>MRGSHHHHHHGSMEQSHQ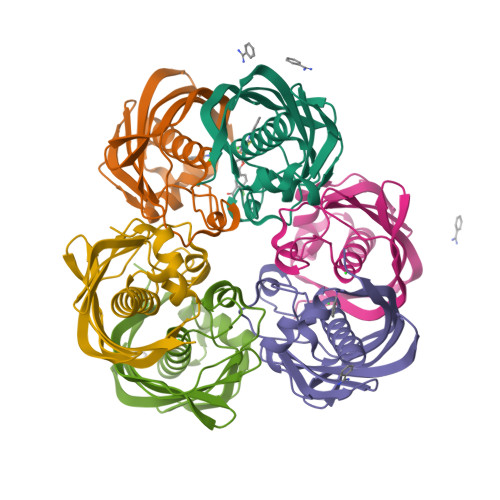NLQSQFFIEHILQILPHRYPMLLVDRITELQANQKIVAYKNITFNEDVFNGHFPNKPIFPGVLIVEGMAQSGGFLAFTSLWGFDPEIAKTKIVYFMTIDKVKFRIPVTPGDRLEYHLEVLKHKGMIWQVGGTAQVDGKVVAEAELKAMIAERE[6x]>SNVPHKSSLPEGIRPGTVLAIRGLVPPNASRFHVNLLCGEEQGSDAALHFNPRLDTSEVVF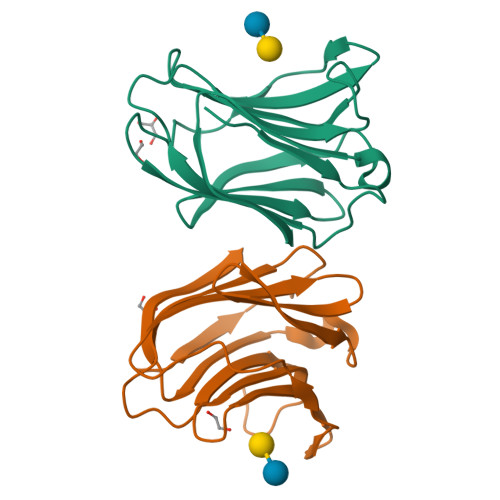NSKEQGSWGREERGPGVPFQRGQPFEVLIIASDDGFKAVVGDAQYHHFRHRLPLARVRLVEVGGDVQLDSVRIF[2x]> L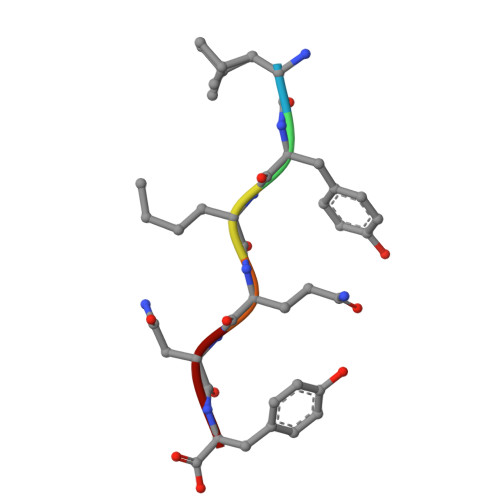YLQNY> GSPSRAEYRNWSKPQCNITGFAPFSKDNSIRLSAGGDIWVTREPYVSCDPDKCYQFALGQGTTLNNGHSNDTVHDRTPYRTLLMNELGVPFHLGTKQVCIAWSSSSCHDGKAWLHVCVTGDDENATASFIYNGRLVDSIGSWSKKILRTQESECVCINGTCTVVMTDGSASGKADTKILFIEEGKIVHTSPLSGSAQHVEECSCYPRYPGVRCVCRDNWKGSNRPIVDINVKDYSIVSSYVCSGLVGDTPRKNDSSSSSHCLDPNNEEGGHGVKGWAFDDGNDVWMGRTISEKLRSGYETFKVIEGWSKPNSKLQINRQVIVDRGNRSGYSGIFSVEGKSCINRCFYVELIRGRKQETEVLWTSNSIVVFCGTSGTYGTGSWPDGADINLMPI

Influenza A virus has two surface glycoproteins, hemagglutinin (HA) and neuraminidase (NA), that act as the major antigens. NA is a type II transmembrane protein that forms a homotetramer. The natural function of NA is to cleave the sialic acids from cellular receptors to facilitate virus release and from newly synthesized HA to prevent virion aggregation. Neuraminidase (NA) of human influenza H3N2 virus has evolved rapidly and been accumulating mutations for more than half-century.

To further examine the structural mechanism of epistasis between K385N and N387K, we determined the crystal structure of NAs from Bil69, SD93, and Mos99 to 1.54 Å, 1.65 Å, and 1.40 Å, respectively. In fact, the double mutant K385N/N387K in Mos99 yielded a WT-like titer, demonstrating that K385N was a permissive mutation for N387K. Flow cytometry analysis showed that N387K decreased the cell surface expression of Mos99 NA, while the addition of K385N restored it. Our results showed that N387K reduced the Tm of Mos99 NA and SD93 NA by around 5 °C. The destabilizing effect of N387K could be partially compensated by K385N. However, K385N alone was not stabilizing, suggesting that the epistasis between K385N and N387K was specific. Asn387 in Mos99 NA is sandwiched by two positively charged residues, Lys385 and Lys389. Consequently, the positively charged mutation N387K would result in an unfavorable electrostatic interaction with Lys385 and Lys389, which explains the destabilizing effect of N387K in Mos99 NA. Nevertheless, K385N removes a positively charged side chain, which enables Lys387 to adapt a different backbone conformation and point away from Lys389 to minimize unfavorable electrostatic interaction. Therefore, our structural analysis explains why K385N is a permissive mutation for N387K and exemplifies how specific epistasis in the natural evolution of human H3N2 NA modulates its structural conformation.> NQCLDVQSRDFVQGVSGGTWVDVVLDHDNCITIVADGKPSFDIRLSKMSMSKFAEYKRYCLQATMSDVTSIVACPGAGDAHNDKSKNHEYICKAVNNDRGWGNGCVLFGKGSMETCGKFECKKKMAGKLVARENVESVVTVHVHGASATDTKGVDTASTAKATITPKASVATLNLNDFGSLEVDCSTDVGMDFGEIVVADMSGKWWIVNKDWFNELALPWSTASTTAEVWQARDRLVEFGWPHAAKQNIYDIGDQEGAVTAAIAQAPMAKWESDKVE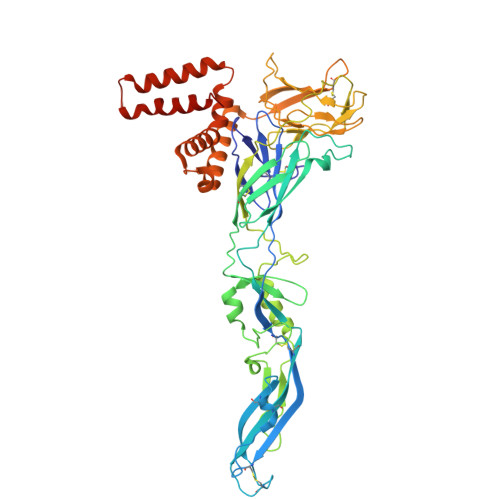LISGILKCKVKLGNLKLRGVTYSMCAQTFTTETRPADTGHGTVAFKVKYVGTDVPCRVPLHIIDSDGGVAAGRVITAHPFVMKQNDYIILEVEPPFGDSKIEIGTGTTKLVEAWHRKGSSIGNAFTATYKGITKLTVLGEHAWDFNSLGGFGASLGKAVHTLFGGVFRVMFGGMGWLTKIFVGAVLVWLGLGAHDKTIATTMILVGSILMYMAVTVGALS>MYRLLNKTAVITGGNSGIGLATAKRFVAEGAYVFIVGRRRKELEQAAAEIGRNVTAVKADVTKLEDLDRLYAIVREQRGSIDVLFANSGAVEQKTLEEITPEHYDRTFDVNVRGLIFTVQKALPLLRDGGSVILTSSVAGVLGLQAHDTYSAAKAAVRSLARTWTTELKGRSIRVNAVSPGAIDTP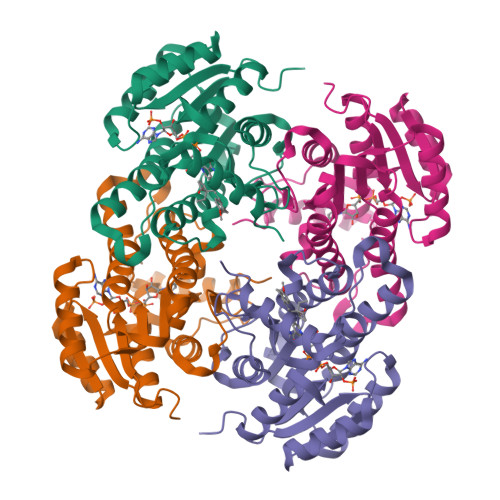SLENNVSTQEEADELRAKAAAATPLGRVGRPEELAAAVLFLASDDSSYVAGIELFVDGGLTQV[2x]>VIQLGRIYLDMLNVYKCLSENISAAIQANGEMVTKQPLIRSMRTVKRETLKLISGWVSRSNDPQMVAENFVPPLLDAVLIDYQRNVPAAREPEVLSTMAIIVNKLGGHITAEIPQIFDAVFECTLNMINKDFEEYPEHRTNFFLLLQAVNSHCFPA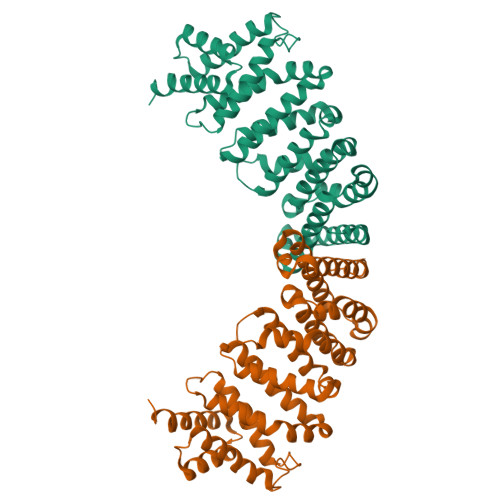FLAIPPTQFKLVLDSIIWAFKHTMRNVADTGLQILFTLLQNVAQEEAAAQSFYQTYFCDILQHIFSVVTDTSHTAGLTMHASILAYMFNLVEEGKISTSLNPGNPVNNQIFLQEYVANLLKSAFPHLQDAQVKLFVTGLFSLNQDIPAFKEHLRDFLVQIKEFAG[2x]>[4x]MGALESLRGNADLAYILSMEPCGHCLIINNVNFCRESGLRTRTGSNIDCEKLRRRFSSLHFMVEVKGDLTAKKMVLALLELARQDHGALDCCVVVILSHGCQ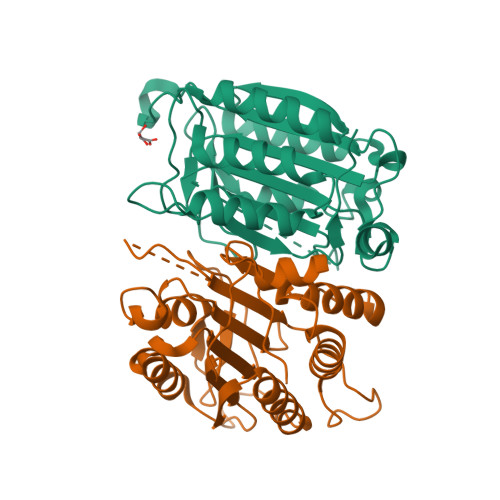ASHLQFPGAVYGTDGCPVSVEKIVNIFNGTSCPSLGGKPKLFFIQASGGEQKDHGFEVASTSPEDESPGSNPEPDATPFQEGLRTFDQLDAISSLPTPSDIFVSYSTFPGFVSWRDPKSGSWYVETLDDIFEQWAHSEDLQSLLLRVANAVSVKGIYKQMPCIVSMLRKKLFFKTS>DLLELTEDMEKEISNALGHGPQDEILSSAFKLRITRGDIQTLKNYHWLNDEVINFYMNLLVERNKKQGYPALHVFSTFFYPKLKSGGYQAVKRWTKGVNLFEQEIILVPIHRKVHWSLVVIDLRKKCLKYLDSMGQKGHRICEILLQYLQDESKTKRNSDLNLLEWTHHSMKPHEIPQQLNGSDCGMFTCKYADYISRDKPITFTQHQMPLFRKKM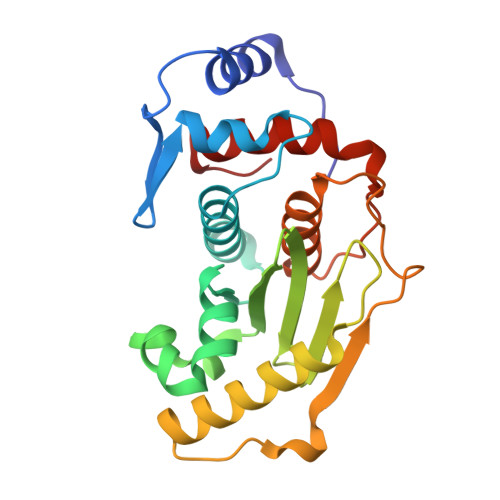VWEILHQQLL[2x]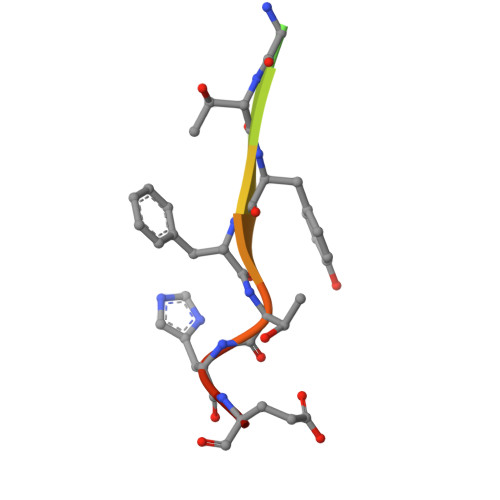> ARHKGTYFTHEA N-({5-[3-(2-amino-4-oxo-4,7-dihydro-1H-pyrrolo[2,3-d]pyrimidin-6-yl)propyl]thiophen-2-yl}carbonyl)-L-glutamic 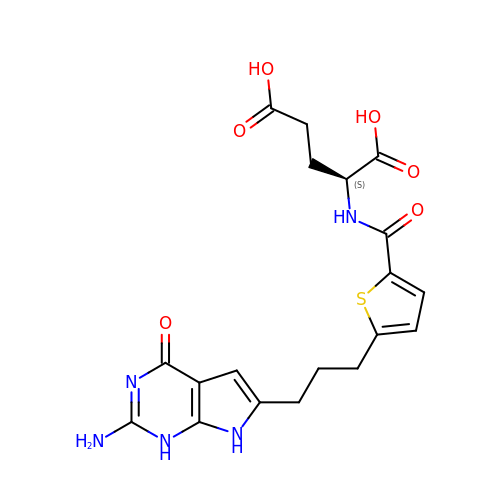acid | C19 H21 N5 O6 S | WMBYSCVMFMNUQV-LBPRGKRZSA-N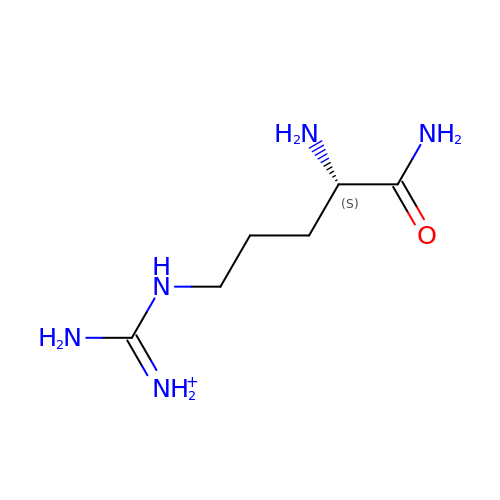ARGININEAMIDE | C6 H16 N5 O | ULEBESPCVWBNIF-BYPYZUCNSA-O3,6-DIHYDROXY-XANTHENE-9-PROPIONIC 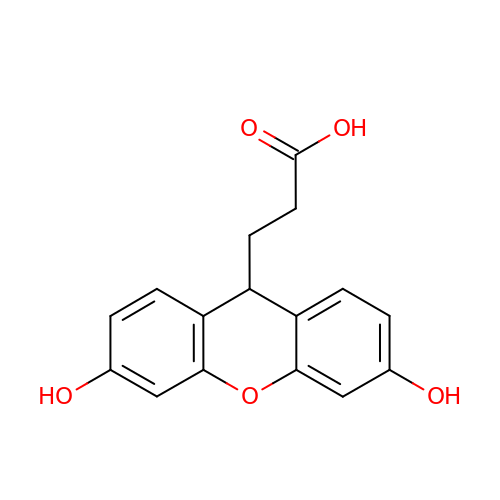ACID | C16 H14 O5 | PFQGLFBMMPZYEU-UHFFFAOYSA-N>DQLDESLRDKVLQLQKGSDTEAQCEVMQEIVDQVLEEDFDSEQLSVLASCLQELFKAHFRGEVLPEEITEESLEESVGKPLYLIFRNLCQMQEDNSSFSLLLDLLSELYQKQPKIGYHLLYYLRASKAAAGKMNLYESFAQATQLGDLHTCLMMDMKACQEDDVRLLCHLTPSIYTEFPDETLRSGELLNMIVAVIDSAQLQELVCHVMMGNLVMFRKDSVLNILIQSLDWETFEQYCAWQLFLAHNIPLETIIPILQHL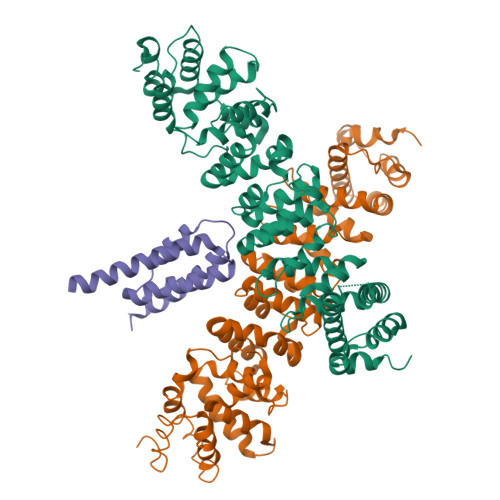KYKEHPEALSCLLLQLRREKPSEEMVKMVLSRPCHPDDQFTTSILRHWCMKHDELLAEHIKSLLIKNNSLPRKRQSLRSSSSKLAQLTLEQILEHLDNLRLNLTNTKQNFFSQTPILQALQHVQASCDEAHKMKFSDLFSLAEEYEDSSTKPPKSRRKAALSSPRSRKNATQPPNAEEESGSSSASEEEDTKPKPTKRKRKGSSAVGSDSD[2x];> PGSAMAKKINDDIKYQLMKEVRRFGQNYERIFILLEEVQGSMKVKRQFVEFTIKEAARFKKVVLIQQLEKALKEIDSHCHLRKVKHMRKR> MTEQQKLTFTALQQRLDSLMLRDRLRFSRRLHGVKKVKNPDAQQAIFQEMAKEIDQAAGKVLLREAARPEITYPDNLPVSQKKQDILEAIRDHQVVIVAGETGSGKTTQLPKICMELGRGIKGLIGHTQPRRLAARTVANRIAEELKTEPGGCIGYKVRFSDHVSDNTMVKLMTDGILLAEIQQDRLLMQYDTIIIDEAHERSLNIDFLLGYLKELLPRRPDLKIIITSATIDPERFSRHFNNAPIIEVSGRTYPVEVRYRPIVEEADDTERDQ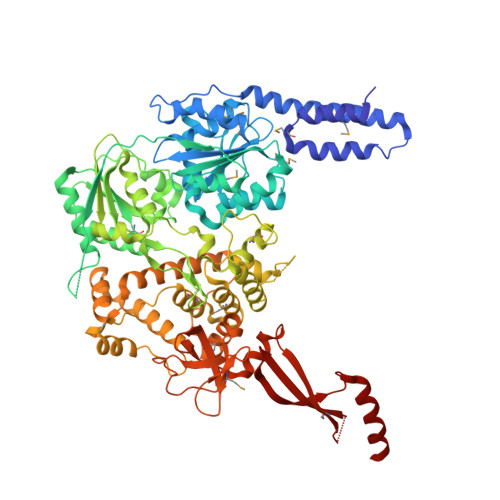LQAIFDAVDELSQESHGDILIFMSGEREIRDTADALNKLNLRHTEILPLYARLSNSEQNRVFQSHSGRRIVLATNVAETSLTVPGIKYVIDPGTARISRYSYRTKVQRLPIEPISQASANQRKGRCGRVSEGICIRLYSEDDFLSRPEFTDPEILRTNLASVILQMTALGLGDIAAFPFVEAPDKRNIQDGVRLLEELGAITTDEQASAYKLTPLGRQLSQLPVDPRLARMVLEAQKHGCVREAMIITSALSIQDPRERPMDKQQASDEKHRRFHDKESDFLAFVNLWNYLGEQQKALSSNAFRRLCRTDYLNYLRVREWQDIYTQLRQVVKELGIPVNSEPAEYREIHIALLTGLLSHIGMKDADKQEYTGARNARFSIFPGSGLFKKPPKWVMVAELVETSRLWGRIAARIDPEWVEPVAQHLIKRTYSEPHWERAQGAVMATEKVTVYGLPIVAARKVNYSQIDPALCRELFIRHALVE> MGPVTLIKDIENQTVLKDNDAVFEIDIKINYPEIKL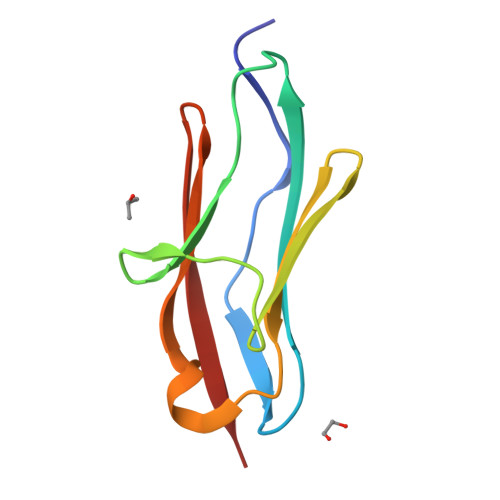SWYKGTEKLEPSDKFEISIDGDRHTLRVKNCQLKDQGNYRLVCGPHIASAKLTVIE Fragaceatoxin C (FraC)11 is a potent haemolysin of the family of actinoporins, defined as a group of ~20 kDa protein toxins produced by sea anemones. Actinoporins are classified as α-helical PFT (α-PFT) because the transmembrane pore is predicted to form an α-helical barrel. The lytic activity of actinoporins on biological membranes is enhanced by the lipid sphingomyelin (SM) and by lipid-phase coexistence. Here we reveal structures of FraC corresponding to four different stages of its activation route, namely the water-soluble form, the lipid-bound form, an assembly intermediate and the transmembrane pore.

The crystal structure of a dimeric form of FraC in two crystal forms at 1.57 and 1.60 Å resolution sheds light on the initial events leading to the assembly of the pore. These two high-resolution crystal structures are virtually identical to each other. Suitable crystals were obtained in the presence of POC (a compound that mimics the lipid headgroup of DOPC and SM) and the detergent dodecyl-β-maltoside (DDM). Two molecules of POC are bound to each protein chain, occupying identical positions to those of the headgroups of lipids L2 and L3 in the crystal structure of both, the transmembrane pore and the DHPC-bound monomer. The protein–protein dimerization surface and the non-covalent interactions observed in the dimer resemble those between residues of the β-core region in the transmembrane pore (rmsd=0.4±0.04 Å). The structure of the dimer reveals a localized and notable conformational change with respect to the monomer (water soluble) at residues 14–17 of the N-terminal region. In the monomeric form of FraC, the side chain of Phe16 is inserted in a hydrophobic cavity of the β-core region. In contrast, during dimerization the residue Val60 of a second protein chain displaces Phe16 from its original position, leading to (i) partial unfolding and increase strain in the peptide bond of Phe16 and its neighbouring residue Leu14, (ii) a displacement of 4.7±0.1 Å of the Cα of Phe16 towards the solvent and (iii) further structural adjustments of Gly15 and Asp17. Because the N-terminal region is glued to the β-core region, partly by interactions between apolar residues, the rearrangement of two large hydrophobic residues (Leu14 and Phe16) may facilitate the detachment of the N-terminal region towards the membrane, a necessary condition to generate the active pore. Second, the serendipitous capture of a dimeric form of FraC exhibiting a similar protein–protein interaction interface to that of the pore, suggests a mechanism initiating the self-assembly and metamorphosis of FraC.

>[4x]SADVAGAVIDGAGLGFDVLKTVLEALGNVKRKIAVGIDNESGKTWTAMNTYFRSGTSDIVLPHKVAHGKALLYNGQKNRGPVATGVVGVIAYSMSDGNTLAVLFSVPYDYNWYSNWWNVRVYKGQKRADQRMYEELYYHRSPFRGDNGWHSRGLGYGLKSRGFMNSSGHAILEIHVTKA> GSHMGSRDHLFKVLVVGDAAVGKTSLVQRYSQDSFSKHYKSTVGVDFALKVLQWSDYEIVRLQLWDIAGLERFTSMTR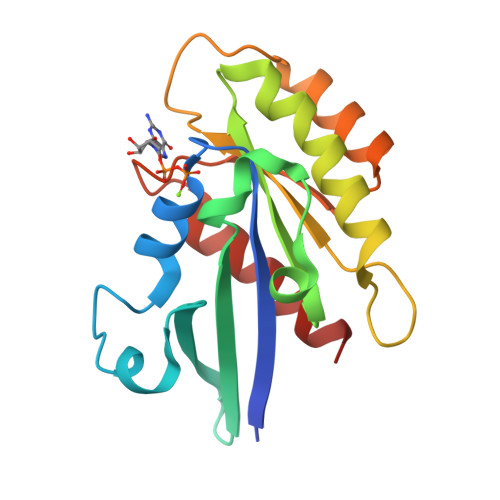LYYRDASAAVIMFDVTNATTFSNSQRWKQDLDSKLTLPNGEPVPALLLANKSDLSPWAVSRDQIDRFSKENGFTGWTETSVKENKNINEAMRVLIEKMMRNS> SMKIPNIGNVMNKFEILGVVGEGAYGVVLKCRHKETHEIVAIKKFKDSEENEEVKETTLRELKMLRTLKQENIVELKEAFRRRGKLYLVFEYVEKNMLELLEEMPNGVPPEKVKSYIYQLIKAIHWCHKNDIVHRDIKPENLLISHNDVLKLCDFGFARNLSEGNNANYDEEVATRWYRSPELLLGAPYGKSVDMWSVGCILGELSDGQPLFPGESEIDQLFTIQKVLGPLPSEQMKLFYSNPRFHGLRFPAVNHPQSLERRYLGILNSVLLDLMKNLLKLDPADRYLTEQCLNHPTFQTQRLL

Here, we present the crystal structures of human CDKL1, CDKL2, CDKL3, and CDKL5, revealing their evolutionary divergence from CDK and mitogen-activated protein kinases (MAPKs), including an unusual αJ helix important for CDKL2 and CDKL3 activity. CDKL family proteins contain a conserved N-terminal kinase domain and variable C termini. The kinase domains of CDKL1, CDKL2, CDKL3, and CDKL5 were crystallized using a phosphomimetic Asp-X-Glu (DXE) substitution and in the presence of identified inhibitors. The CDKL structures all contain broad spectrum ATP-competitive inhibitors that bind to the kinase hinge region via 3 hydrogen bonds.

By contrast, the CDKL1, CDKL3, and CDKL5 structures displayed characteristics of active kinases. Inhibitor ASC67 was designed as an affinity reagent (Statsuk et al., 2008) and was among the top screening hits for all CDKLs tested. Its nitrile H bonded with the catalytic lysines of CDKL3 and CDKL5. Catalytic site interactions may help support the active conformation of these kinases. Instead, CDKL2 and CDKL3 showed an unusual amphipathic helix, αJ, while the constructs for CDKL1 and CDKL5 were truncated and lacked this region. Notably, deleting the αJ region reduced the activities of CDKL2 and CDKL3, whereas CDKL1 and CDKL5 were largely unchanged. Disrupting CDKL5 causes Rett syndrome, a neurodevelopmental disorder that exhibits early-onset seizures, mental retardation, and autism (Castrén et al., 2011, Kilstrup-Nielsen et al., 2012). CDKL5 mutations, most occurring in the kinase domain, are linked to neurological disorders, including epilepsy, atypical Rett syndrome, and autism. To this end, we found that GFP-tagged human CDKL5 localizes at the basal body, as well as ciliary tip in ciliated RPE-1 cells. We chose to model three pathogenic CDKL5 missense mutations (G20R, P180L, and L220P) present in patients with epileptic encephalopathy, severe mental retardation, developmental delay, or spasms (Kilstrup-Nielsen et al., 2012).> MNRAFSRKKDKTWMHTPEALSKHFIPYNAKFLGSTEVEQPKGTEVVRDAVRKLKFARHIKKSEGQKIPKVELQISIYGVKILEPKTKEVQHNCQLHRISFCADDKTDKRIFTFICK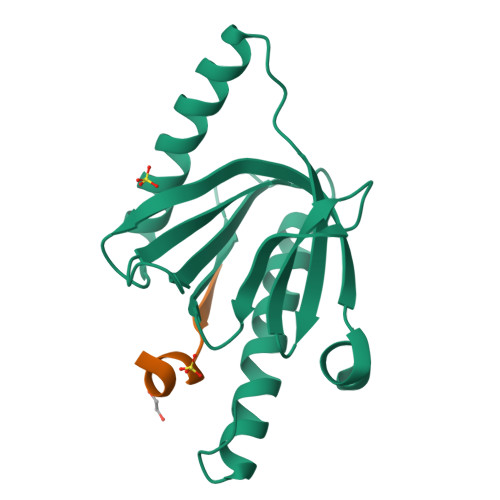DSESNKHLCYVFDSEKCAEEITLTIGQAFDLAYRKFLESGGKDVETRKQIAG;> NGYENPTYKFFE>MAAPLPEGVSAEAMSSALDRFARIVGADWVFTEDKITPYEDPYTISNDETEHRPYAAVAPASTEEVQEIVRVANEFGVPLWPVSRGKNFAYGGAAPVMSGTVVLDMNRMNRILEVNEEFGYALVEPGVSYFELYDYIQEKGLKLWIDVPDVGWGSVVGNALDHGIGYTPYGDHFAMQCGMEVVLPNGEVVRTGMGAMPGNNTWQLFKYGYGPYVDGIFSQSNFGVVTKMGIWLMPEPAGYRPYLITFENEDDIETVTERLRPLKVAGVIQNGATVRSLVLDAAITRTKSQYYDGDGPIPPSVAKTMMADLDLGMWNFCGALYGPPPVMDTLWTAIRDSFADIPGVKFYFPEDRRHKVDLLLHRAETMKGVPKLTEFNFLNWDGGGGHVGFSPVSPITGKDAIKQYNMVSSRVREYGFDYMGLLAIGWRDLHHVTVIVYDKTDPDERKKLDELFNILVDEAAAEGYGEYRTHIRYMDRIAKTYSWNDNALWKMHETIKDALDPNGILAPGKSGIWGKNRRKA[2x]

Enzymes of the vanillyl alcohol oxidase/p-cresol methyl hydroxylase (VAO/PCMH) superfamily are found across all kingdoms where they perform a range of metabolic functions. These flavoproteins share a conserved FAD-binding domain and a more variable substrate-binding domain that enables interactions with a range of substrates. One of these, the 4-phenol oxidases/dehydrogenases, catalyzes the oxidation of para-substituted phenolic compounds. A fundamental distinction is that the oxidases efficiently react with oxygen producing hydrogen peroxide whereas the dehydrogenases hardly react with oxygen and typically employ other proteins, such as cytochrome c, as acceptors.

Pro151 was substituted with isoleucine and valine to mimic the N5 environment of EUGHs. We found that P151V and P151I can operate with oxygen although they are 10- to 40-fold less efficient compared to using 2,6-dichlorophenolindophenol as co-substrate. The crystal structures of the six P151 mutants were also solved. They are closely similar to the wild-type regarding the substrate-binding residues whereas loop 150-153 locally undergoes localized rearrangements, with each mutant adopting a distinct conformation. In general, the oxidase-active variants (P151L, P151G, P151I, P151V) all adopt the trans conformation that slightly shifts the amino acid at position 151 away from the flavin. The analysis revealed a consistent pattern: in the oxidase mutants, the 150-153 loop conformations create tunnels that lead to the flavin re side. The ability of nsVAO to use oxygen as electron acceptor thereby aligns with the oxidase activity observed for the P151V mutant of VAD.> AELPQMTQQLNSDDMQEQLSATVKFRQILSREHRPPIDVVIQAGVVPRLVEFMRENQPEMLQLEAAWALTNIASGTSAQTKVVVDADAVPLFIQLLYTGSVEVKEQAIWALGNVAGDSTDYRDYVLQCNAMEPILGLFNSNKPSLIRTATWTLSNLCRGKKPQPDWSVVSQALPTLAKLIYSMDTETLVDACWAISYLSDGPQEAIQAVIDVRIPKRLVELLSHEST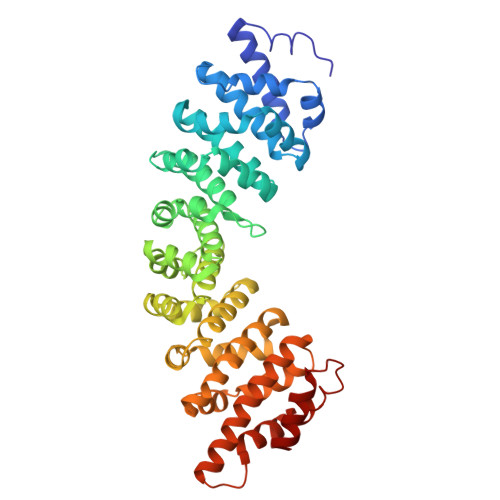LVQTPALRAVGNIVTGNDLQTQVVINAGVLPALRLLLSSPKENIKKEACWTISNITAGNTEQIQAVIDANLIPPLVKLLEVAEYKTKKEACWAISNASSGGLQRPDIIRYLVSQGCIKPLCDLLEIADNRIIEVTLDALENILKMGEADKEARGLNINENADFIEKAGGMEKIFNCQQNENDKIYEKAYKIIETYF>[2x]MSKFTWKELIQLGSPSKAYESSLACIAHIDMNAFFAQVEQMRCGLSKEDPVVCVQWNSIIAVSYAARKYGISRMDTIQEALKKCSNLIPIHTAVFKKGEDFWQYHDGCGSWVQDPAKQISVEDHKVSLEPYRRESRKALKIFKSACDLVERASIDEVFLDLGRICFNMLMFDNEYELTGDLKLKDALSNIREAFIGGNYDINSHLPLIPEKIKSLKFEGDVFNPEGRDLITDWDDVILALGSQVCKGIRDSIKDILGYTTSCGLSSTKNVCKLASNYKKPDAQT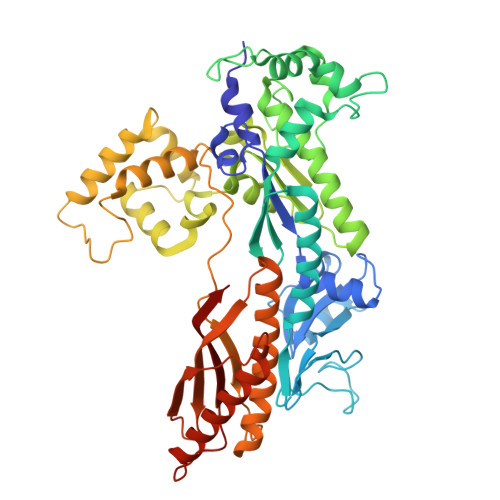IVKNDCLLDFLDCGKFEITSFWTLGGVLGKELIDVLDLPHENSIKHIRETWPDNAGQLKEFLDAKVKQSDYDRSTSNIDPLKTADLAEKLFKLSRGRYGLPLSSRPVVKSMMSNKNLRGKSCNSIVDCISWLEVFCAELTSRIQDLEQEYNKIVIPRTVSISLKTKSYEVYRKSGPVAYKGINFQSHELLKVGIKFVTDLDIKGKNKSYYPLTKLSMTITNFDIIDLQK> MYLPSMKHSLPLLAALVLAACSSTNTLPAGKTPADNIETADLSASVPTRPAEPERKTLADYGGYPSALDAVKQKNDAAVAAYLENAGDSAMAENVRNEWLKSLGARRQWTLFAQEYAKLEPAGRAQEVECYADSSRNDYTRAAELVKNTGKLPSGCTKLLEQAAASGLLDGNDAWRRVRGLLAGRQTTDARNLAAALGSPFDGGTQGSREYALLNVIGKEARKSPNAAALLSEMESGLSLEQRSFAWGVLGHYQSQNLNVPAALDYYGKVADRRQLTDDQIEWYARAALRARRWDELASVISHMPEKLQKSPTWLYWLARSRAATGNTQEAEKLYKQAAATGRNFYAVLAGEELGRKIDTRNNVPDAGKNSVRRMAEDGAVKRALVLFQNSQSAGDAKMR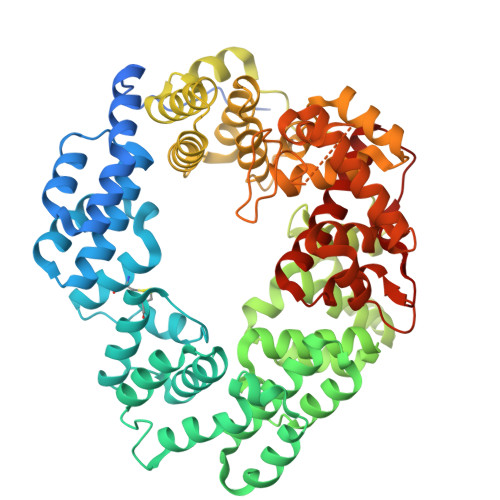RQAQAEWRFATRGFDEDKLLTAAQTAFDHGFYDMAVNSAERTDRKLNYTLRYISPFKDTVIRHAQNVNVDPAWVYGLIRQESRFVIGAQSRVGAQGLMQVMPATAREIAGKIGMDAAQLYTADGNIRMGTWYMADTKRRLQNNEVLATAGYNAGPGRARRWQADTPLEGAVYAETIPFSETRDYVKKVMANAAYYAALFGAPHIPLKQRMGIVPAR> AGAGCGUUGCGUCCGAAAGUCGCC;> GCGA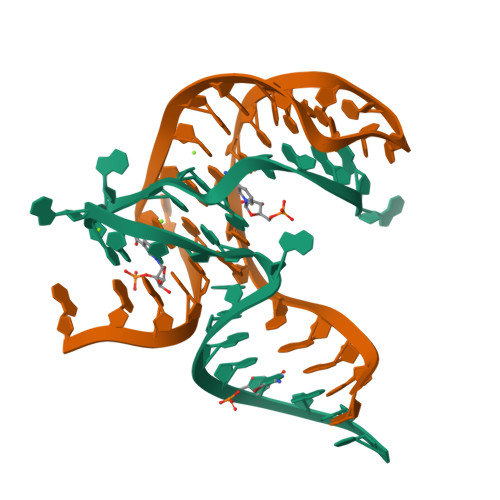CACGGCUCUUUAAAAACAAAAGGAGA>[2x]MKFAEHLTAHITPEWRKQYINYEEMKAMLYAAIEQSPSAELVEREMVTRYFAKFDEEFFHYCDKELAKINTFYSEKMAEATRKYGSLRSELTEALEMGHPKKLPAWKRRTPLGKKNVPARKIQDLKLAFSEFYLGLILLQNYQNLNFTGFRKILKKHDKLLSVDYGARWRTDHVEAAHFYTNKDIDRLIQETEQAVTQDIEGGDRQRAMKRLRVPPLGEQQSPWTTFKVGLFSGAFVVLFITVVIAAMFYGFGENWRAGMRMFRAPFLIIECLFLWGVNVYGWRSSGVNHVLIFELDPRNHLSEQNIMEVASVFGVIWAC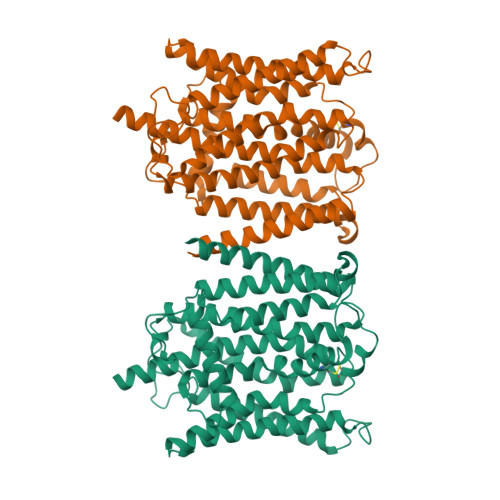CVLSYIFCDPLGIPQYAAPLCLYTLMAAFLLNPTKTFHHEARFWAIRILIRVIMAPFCFVNFADFWLADQLNSMVPAFLDIPFLICFFGRSPTWHKAGKAASHCVEYVSLLHPIVAIMPAYFRFAQCIRRYRDTKESFPHLVNAAKYATSFFVVIFAHKYHTTTDTYPLSKENPWFYCWITAAIFSSCYAYTWDIKMDWGLFDSKAGDNRFLREEIVYSSTWFYYFGIIEDLILRFSWTLSMSLIEAGYIEGDVMMTILSPLEVFRRFIWNYFRLENEHLNNVAKFRAVRDISVAPMDCSDQTTILRMMDETDGVLNRRRGKAAGGKSATKKNKQEQRLLLQGESIEDLCS> MSTMSTPAAEQRKLVEQLMGRDFSFRHNRYSHQKRDLGLHDPKICKSYLVGECPYDLFQGTKQSLGKCPQMHLTKHKIQYEREVKQGKTFPEFEREYLAILSRFVNECNGQISVALQNLKHTAEERMKIQQVTEELDVLDVRIGLMG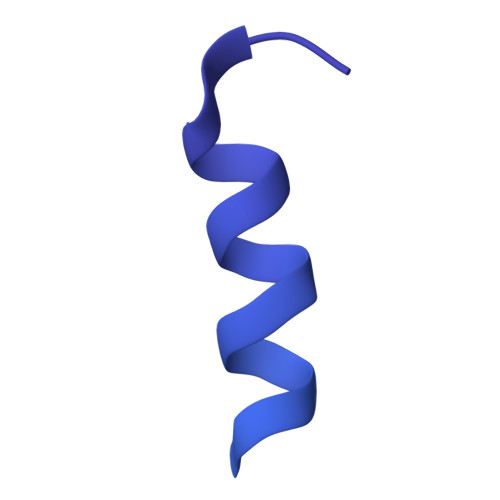QEIDSLIRADEVSMGMLQSVKLQELISKRKEVAKRVRNITENVGQSAQQKLQVCEVCGAYLSRLDTDRRLADHFLGKIHLGYVKMREDYDRLMKNNRTTNASKTATTLPGRRFV ethyl 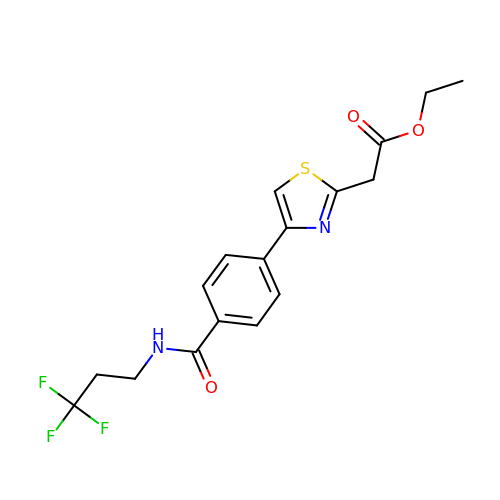2-[4-[4-[3,3,3-tris(fluoranyl)propylcarbamoyl]phenyl]-1,3-thiazol-2-yl]ethanoate | C17 H17 F3 N2 O3 S | BTOQSHVHCYLPJO-UHFFFAOYSA-N>[2x]MSEFSQTVPELVAWARKNDFSISLPVDRLSFLLAVATLNGERLDGEMSEGELVDAFRHVSDAFEQTSETIGVRANNAINDMVRQRLLNRFTSEQAEGNAIYRLTPLGIGITDYYIRQREFSTLRLSMQLSIVAGELKRAADAAEEGGDEFHWHRNVYAPLKYSVAEIFDSIDLTQRLMDEQQQQVKDDIAQLLNKDWRAAISSCELLLSET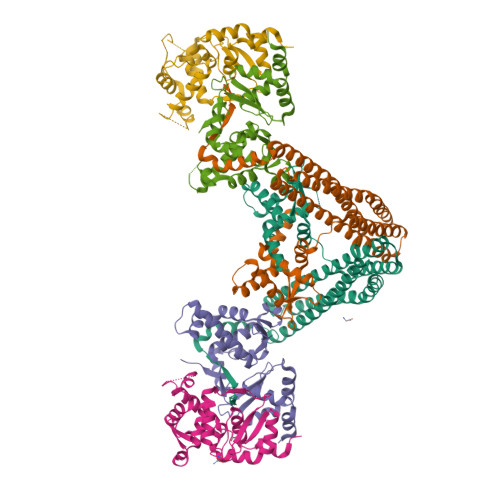SGTLRELQDTLEAAGDKLQANLLRIQDATMTHDDLHFVDRLVFDLQSKLDRIISWGQQSIDLWIGYDRHVHKFIRTAIDMDKNRVFAQRLRQSVQTYFDEPWALTYANADRLLDMRDEEMALRDEEVTGELPEDLEYEEFNEIREQLAAIIEEQLAVYKTRQVPLDLGLVVREYLSQYPRARHFDVARIVIDQAVRLGVAQADFTGLPAKWQPINDYGAKVQAHVIDKY;>[4x]MSSTNIEQVMPVKLAQALANPLFPALDSALRSGRHIGLDELDNHAFLMDFQEYLEEFYARYNVELIRAPEGFFYLRPRSTTLIPRSVLSELDMMVGKILCYLYLSPERLANEGIFTQQELYDELLTLADEAKLLKLVNNRSTGSDVDRQKLQEKVRSSLNRLRRLGMVWFMGHDSSKFRITESVFRFGADVRAGDDPREAQRRLIRDGEAMPIENHLQLNDETEENQPDSGEEE> MEEECRVLSIQSHVVRGYVGNRAATFPLQVLGFEVDAVNSVQFSNHTGYSHWKGQVLNSD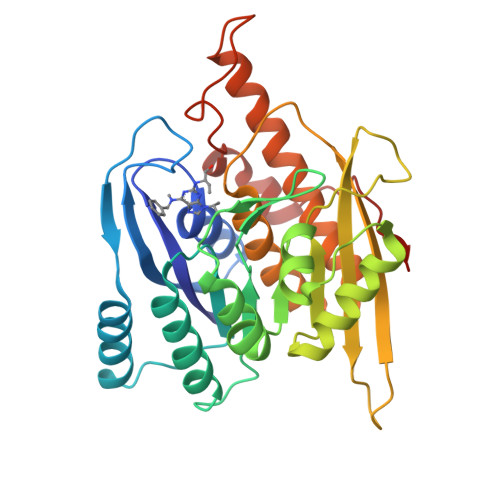ELQELYDGLKLNHVNQYDYVLTGYTRDKSFLAMVVDIVQELKQQNPRLVYVCDPVMGDQRNGEGAMYVPDDLLPVYREKVVPVADIITPNQFEAELLTGRKIHSQEEALEVMDMLHSMGPDTVVITSSNLLSPRGSDYLMALGSQRTRAPDGSVVTQRIRMEMHKVDAVFVGTGDLFAAMLLAWTHKHPNNLKVACEKTVSAMHHVLQRTIKCAKAKSGEGVKPSPAQLELRMVQSKKDIESPEIVVQATVL>GPLGSLVAIQAELTKSQETIGSLNEEIEQYKGT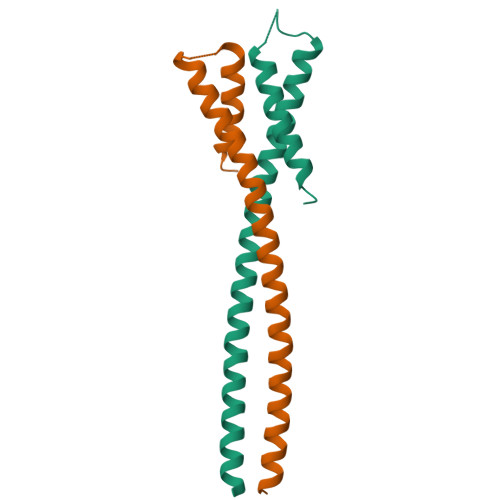VSTLEIEREFYFNKLRDIEILVHTTQDLINEGVYKFNDETITGHGNGNGGALLRFVKKVESILYATAEGFEMN[2x]>[2x]SNAMNFNKLKFGATIGIIGGGQLGKMMAQSAQKMGYKVVVLDPSEDCPCRYVAHEFIQAKYDDEKALNQLGQKCDVITYEFENISAQQLKLLCEKYNIPQGYQAIQLLQDRLTEKETLKSAGTKVVPFISVKESTDIDKAIETLGYPFIVKTRFGGYDGKGQVLINNEKDLQEGFKLIETSECVAEKYLNIKK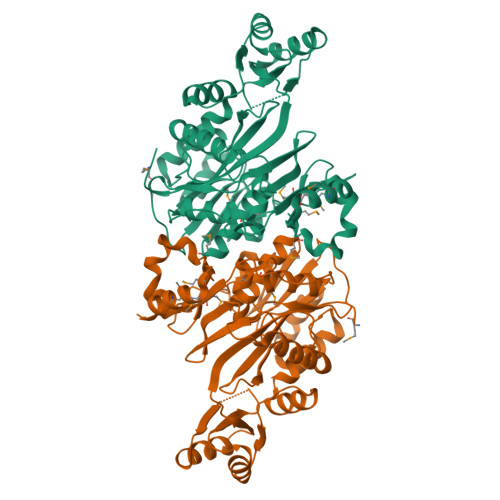EVSLTVTRGNNNQITFFPLQENEHRNQILFKTIVPARIDKTAEAKEQVNKIIQSIHFIGTFTVEFFIDSNNQLYVNEIAPRPHNSGHYSIEACDYSQFDTHILAVTGQSLPNSIELLKPAVMMNLLGKDLDLLENEFNEHPEWHLHIYGKSERKDSRKMGHMTVLTNDVNQTEQDMYAKFEGSN> MSRPLSDQEKRKQISVRGLAGVENVTELKKNFNRHLHFTLVKDRNVATPRDYYFALAHTVRDHLVGRWIRTQQHYYEKDPKRIYYLSLEFYMGRTLQNTMVNLALENACDEATYQLGLDMEELEEIEEDAGLGNGGLGRLAACFLDSMATLGLAAYGYGIRYEFGIFNQKISGGWQMEEADDWLRYGNPWEKARPEFTLPVHFYGHVEHTSQGAKWVDTQVVLAMPYDTPVPGYRNNVVNTMRLWSAKAPNDFNLKDFNVGGYIQAVLDRNLAENISRVLYPNDNFFEGKELRLKQEYFVVAATLQD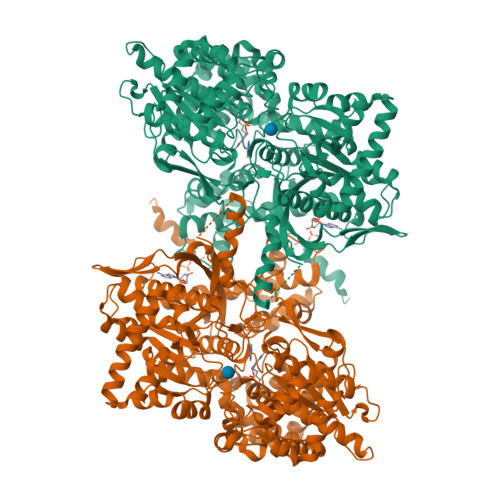IIRRFKSSKFGCRDPVRTNFDAFPDKVAIQLNDTHPSLAIPELMRILVDLERMDWDKAWDVTVRTCAYTNHTVLPEALERWPVHLLETLLPRHLQIIYEINQRFLNRVAAAFPGDVDRLRRMSLVEEGAVKRINMAHLCIAGSHAVNGVARIHSEILKKTIFKDFYELEPHKFQNKTNGITPRRWLVLCNPGLAEVIAERIGEDFISDLDQLRKLLSFVDDEAFIRDVAKVKQENKLKFAAYLEREYKVHINPNSLFDIQVKRIHEYKRQLLNCLHVITLYNRIKREPNKFFVPRTVMIGGKAAPGYHMAKMIIRLVTAIGDVVNHDPAVGDRLRVIFLENYRVSLAEKVIPAADLSEQISTAGTEASGTGNMKFMLNGALTIGTMDGANVEMAEEAGEENFFIFGMRVEDVDKLDQRGYNAQEYYDRIPELRQVIEQLSSGFFSPKQPDLFKDIVNMLMHHDRFKVFADYEDYIKCQEKVSALYKNPREWTRMVIRNIATSGKFSSDRTIAQYAREIWGVEPSRQRLPAPDEAI> MFGTTRVWRNTFLTKSVATPPISVIRTGPKWWADPERMVRQKLMYFTLGVDQLPLRRTAVIQKDLHRFHMCKPPPRIGDTTGYKRSRAAQLTTWYRRIQYQEYHLQHLFTRHVWGLVRAYPGNTTKI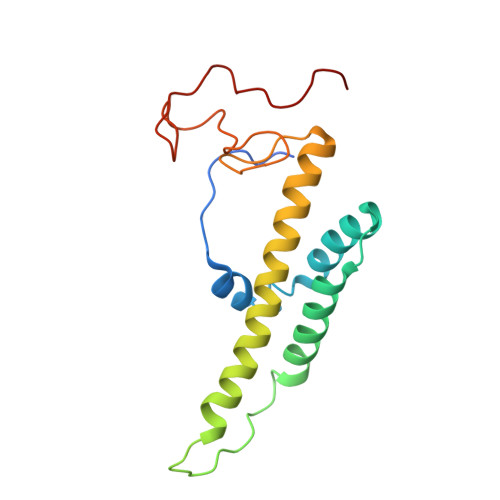QGKADDGYVGYDSVPYHRYNRTPLPFPAREIYGRRE>MASWSHPQFEKMGMLEARELLCERDERTLFSGLSFTLNAGEWVQITGSNGAGKTTLLRLLTGLSRPDAGEVLWQGQPLHQVRDSYHQNLLWIGHQPGIKTRLTALENLHFYHRDGDTAQCLEALAQAGLAGFEDIPVNQLSAGQQRRVALARLWLTRATLWILDQPFTAIDVNGVDRLTQRMAQHTEQGGIVILTTHQPLNVAESKIRRISLTQTRAA[2x];>MMFWRIFRLELRVAFRHSAEIANPLWFFLIVITLFPLSIGPEPQLLARIAPGIIWVAALLSSLLALERLFRDDLQDGSLEQLMLLPLPLPAVVLAKVMAHWMVTGLPLLILSPLVAMLLGMDVYGWQVMALTLLLGTPTLGFLGAPGVALTVGLKRGGVLLSILVLPLTIPLLIFATAAMDAASMHLPVDGYLAILGALLAGTATLSPFATAAALRISIQ[2x];> MWKTLHQLAIPPRLYQICGWFIPWLAIASVVVLTVGWIWGFGFAPADYQQGNSYRIIYLHVPAAIWSMGIYASMAVAAFIGLVWQMKMANLAVAAMAPIGAVFTFIALVTGSAWGKPMWGTWWVWDARLTSELVLLFLYVGVIALWHAFDDRRLAGRAAGILVLIGVVNLPIIHYSVEWWNTLHQGSTRMQQSIDPAMRSPLRWSIFGFLLLSATLTLMRMRNLILLMEKRRPWVSELILKRGRK;> MTPAFASWNEFFAMGGYAFFVWLAVVMTVIPLVVLVVHSVMQHRAILRGVAQQRAREARLRAAQQQEAA

Here we report cryo-electron microscopic structures of the heme translocation complex CcmABCD from E. coli, alone and bound to the heme chaperone CcmE. CcmABCD forms a heterooctameric complex centered around the ABC transporter CcmAB that does not by itself transport heme. Our data suggest that the complex flops a heme group from the inner to the outer leaflet at its CcmBC interfaces, driven by ATP hydrolysis at CcmA. A conserved heme-handling motif (WxWD) at the periplasmic side of CcmC rotates the heme by 90° for covalent attachment to the heme chaperone CcmE that we find interacting exclusively with the CcmB subunit.

As anticipated, the single point mutation in the nucleotide-binding site of CcmA locked the transporter in a closed conformation, shortening the distance between the centers of mass for the two CcmA subunits from 36 Å to 29.4 Å. From the inward-open state of the nucleotide-free Ccm(AB)2 heterotetramer, the E154QA variant switched to a fully closed configuration with no internal cavity of sufficient size to accommodate a cargo molecule of the size of a heme cofactor. No heme was bound in this sample, and we obtained one data set that contained CcmA without and one with bound ATP, with only minor changes to the overall conformation of the complex. The overall conformational changes in the different states of CcmA were subtle, and the nucleotide-free wild-type structure showed the same conformation of the P-loop as the nucleotide-free E154QA variant, although the latter switched the transporter into its closed state. Unexpectedly, the overall stoichiometry of the CcmABCD changed for the E154QA variant, in that the closure of the core ABC transporter Ccm(AB)2 consistently led to the loss of one copy of CcmCD, resulting in a Ccm(E154QAB)2CD complex. This fundamental change in quaternary structure led to a structural asymmetry of the two CcmB protomers. The inner protomer of CcmB largely retained its open-state conformation, as was the case for the adjacent, remaining copies of CcmC and CcmD. The outer protomer, however, now unrestrained by interactions with CcmCD, underwent a conformational change that most strongly affected the cytoplasmic termini of its transmembrane helices hI and hV. In the outer protomer of the E154QA variant complex, the cytoplasmic ends of both helices moved outward from the core of the CcmB dimer, by 7.0 Å in the case of hI and 8.1 Å for hV. This latter shift would have caused a significant clash with transmembrane helix hIV of CcmC and is therefore the likely reason for the dissociation of the second copy of CcmCD from a heterooctameric Ccm(ABCD)2 complex.> MFQSTEQALAVAYWMFEQQPGPRSSTAMVIDSLRERFDRRFIERLPSGLSPHEWQAQAVMTVRFAQRQLAAHPLELAVVRAEFARGRDFVLGLAALRDWLKPAAGPIEQRAALALLMRMFRRPPSSIREI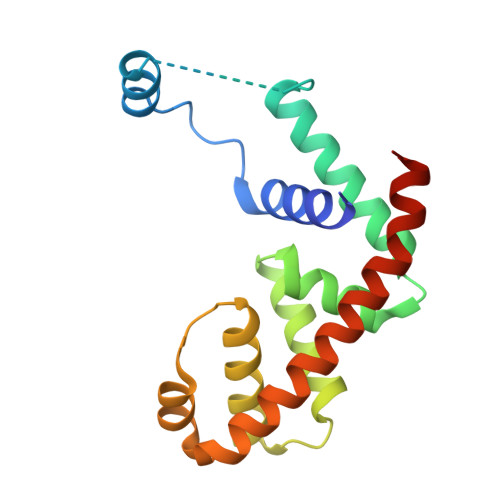ERLSGLSKSTLHRWDKEWRERVAALLRQALLRLEEPMAQVGIVCEH>MAKKTSSKGKLPPGPSPLPVLGNLLQMDRKGLLRSFLRLREKYGDVFTVYLGSRPVVVLCGTDAIREALVDQAEAFSGRGKIAVVDPIFQGYGVIFANGERWRALRRFSLATMRDFGMGKRSVEERIQEEARCLVEELRKSKGALLDNTLLFHSITSNIICSIVFGKRFDYKDPVFLRLLDLFFQSFSLISSFSSQVFELFSGFLKYFPGTHRQIYRNLQEINTFIGQSVEKHRATLDPSNPRDFIDVYLLRMEKDKSDPSSEFHHQNLILTVLSLFFAGTETTST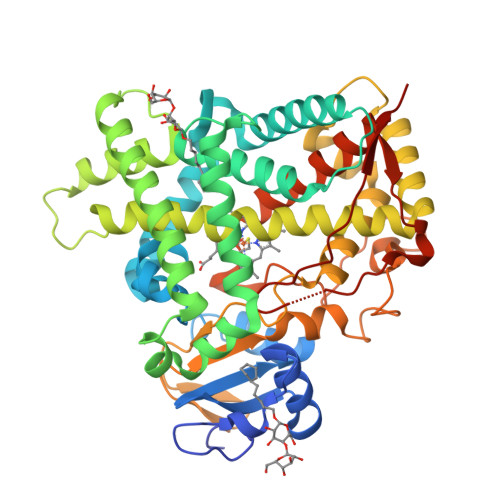TLRYGFLLMLKYPHVTERVQKEIEQVIGSHRPPALDDRAKMPYTDAVIHEIQRLGDLIPFGVPHTVTKDTQFRGYVIPKNTEVFPVLSSALHDPRYFETPNTFNPGHFLDANGALKRNEGFMPFSLGKRICLGEGIARTELFLFFTTILQNFSIASPVPPEDIDLTPRESGVGNVPPSYQIRFLARHHHH[2x]> MKTLVHVASVEKGRSYEDFQKVYNAIALKLREDDEYDNYIGYGPVLVRLAWHTSGTWDKHDNTGGSYGGTYRFKKEFNDPSNAGLQNGFKFLEPIHKEFPWISSGDLFSLGGVTAVQEMQGPKIPWRCGRVDTPEDTTPDNGRLPDADKDADYVRTFFQRLNMNDREVVALMG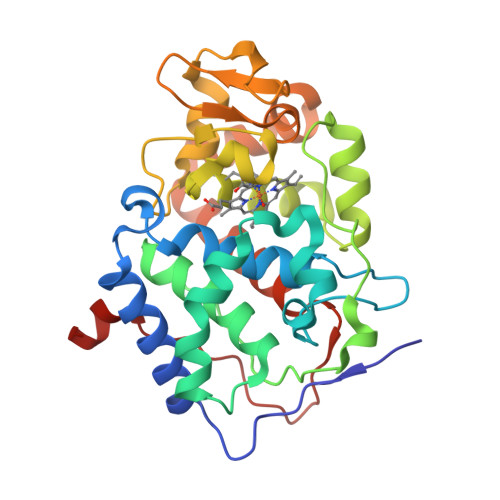AHALGKTHLKNSGYEGPWGAANNVFTNEFYLNLLNEDWKLEKNDANNEQWDSKSGYMMLPTDYSLIQDPKYLSIVKEYANDQDKFFKDFSKAFEKLLENGITFPKDAPSPFIFKTLEEQGL In Gram-negative bacteria, the full Dpp transporter is composed of five subunits: two integral membrane proteins (DppB and DppC) that form a translocation pathway for substrates; two ATPases (DppD and DppF) that bind and hydrolyze ATP during transport and a periplasm-localized SBP (DppA) for substrate capture. The Dpp transporter is primarily responsible for importing dipeptides but also capable of inefficiently importing tri- and tetrapeptides into the cell. Different from those structurally and mechanistically well-characterized ABC exporters that solely consist of two variable transmembrane domains (TMDs) and two highly conserved nucleotide-binding domains (NBDs), the ABC peptide importers require an additional substrate-binding protein (SBP) that captures peptide substrates and delivers them to the translocator for function. Unlike the reported heterotrimeric Mycobacterium tuberculosis DppBCD translocator, the E. coli DppBCDF translocator is a heterotetramer, with a [4Fe-4S] cluster at the C-terminus of each ATPase subunit.

The DppBCDF structure was determined to a global resolution of 3.2 Å. In the final model, except 30 residues, i.e., the periplasmic “scoop motif” region that connects transmembrane (TM) helix TM1 with α3 short helix in DppB, other residues in the DppBCDF complex are unambiguously resolved. The DppBCDF translocator assembles to form a rare heterotetramer with DppB and DppC specifically interacting with DppD and DppF, respectively, exhibiting a pseudo-dimeric symmetry perpendicular to the membrane plane. In the complex, TM helices (TM3, TM4, TM5 and TM6) of both DppB and DppC converge to form a substrate translocation pathway, yet its periplasmic substrate entrance is occluded via hydrophobic interactions. However, on the cytoplasmic side, TM helices (TM3, TM4, TM5 and TM6) of DppB are well separated apart from those of DppC, generating an inverted “V-shaped” substrate translocation pathway open to the cytoplasm. In line with the inward-facing conformation of the two TMDs, the two NBDs, DppD and DppF, also adopt an open conformation with no bound nucleotides observed at the interface. Apparently, the current structure snapshots an inward-facing resting state of the DppBCDF translocator. Notably, the two ATPases, DppD and DppF, in the complex, each binds a [4Fe-4S] cluster via their respective C-terminal domain, consistent with the crystal structure of the isolated DppD from Gram-negative bacteria Thermoanaerobacter tengcongensis. Consistent with our structural findings, DppBCDF has essentially no ATPase activity, even in the presence of dipeptide substrates such as Ala-Ala (AA). In the resting state, the substrate translocation pathway of DppBCDF is inward-facing open to the cytoplasm, sealing the membrane.

> MLQFILRRLGLVIPTFIGITLLTFAFVHMIPGDPVMIMAGERGISPERHAQLLAELGLDKPMWQQYLHYIWGVMHGDLGISMKSRIPVWEEFVPRFQATLELGVCAMIFATAVGIPVGVLAAVKRGSIFDHTAVGLALTGYSMPIFWWGMMLIMLVSVHWNLTPVSGRVSDMVFLDDSNPLTGFMLIDTAIWGEDGNFIDAVAHMILPAIVLGTIPLAVIVRMTRSSMLEVLGEDYIRTARAKGLTRMRVIIVHALRNAMLPVVTVIGLQVGTLLAGAILTETIFSWPGLGRWLIDALQRRDYPVVQGGVLLVATMIILVNLLVDLLYGVVNPRIRHKK;> MSQVTENKVISAPVPMTPLQEFWHYFKRNKGAVVGLVYVVIVLFIAIFANWIAPYNPAEQFRDALLAPPAWQEGGSMAHLLGTDDVGRDVLSRLMYGARLSLLVGCLVVVLSLIMGVILGLIAGYFGGLVDNIIMRVVDIMLALPSLLLALVLVAIFGPSIGNAALALTFVALPHYVRLTRAAVLVEVNRDYVTASRVAGAGAMRQMFINIFPNCLAPLIVQASLGFSNAILDMAALGFLGMGAQPPTPEWGTMLSDVLQFAQSAWWVVTFPGLAILLTVLAFNLMGDGLRDALDPKLKQ;> MALLNVDKLSVHFGDESAPFRAVDRISYSVKQGEVVGIVGESGSGKSVSSLAIMGLIDYPGRVMAEKLEFNGQDLQRISEKERRNLVGAEVAMIFQDPMTSLNPCYTVGFQIMEAIKVHQGGNKSTRRQRAIDLLNQVGIPDPASRLDVYPHQLSGGMSQRVMIAMAIACRPKLLIADEPTTALDVTIQAQIIELLLELQQKENMALVLITHDLALVAEAAHKIIVMYAGQVVETGDAHAIFHAPRHPYTQALLRALPEFAQDKERLASLPGVVPGKYDRPNGCLLNPRCPYATDRCRAEEPALNMLADGRQSKCHYPLDDAGRPTL;> MSTQEATLQQPLLQAIDLKKHYPVKKGMFAPERLVKALDGVSFNLERGKTLAVVGESGCGKSTLGRLLTMIEMPTGGELYYQGQDLLKHDPQAQKLRRQKIQIVFQNPYGSLNPRKKVGQILEEPLLINTSLSKEQRREKALSMMAKVGLKTEHYDRYPHMFSGGQRQRIAIARGLMLDPDVVIADEPVSALDVSVRAQVLNLMMDLQQELGLSYVFISHDLSVVEHIADEVMVMYLGRCVEKGTKDQIFNNPRHPYTQALLSATPRLNPDDRRERIKLSGELPSPLNPPPGCAFNARCRRRFGPCTQLQPQLKDYGGQLVACFAVDQDENPQR The snRNA activating protein complex (SNAPc) exclusively recognizes the proximal sequence element (PSE) at snRNA promoters and recruits RNA polymerase II or III to initiate transcription. The vertebrate SNAPc consists of five subunits: SNAP190 (SNAPC4, PTFα), SNAP50 (SNAPC3, PTFβ), SNAP45 (SNAPC2, PTFδ), SNAP43 (SNAPC1, PTFγ), and SNAP19 (SNAPC5). The partial complex, termed mini-SNAPc, is composed of N-terminal third part of SNAP190, SNAP50, and SNAP43, and is fully functional for PSE-binding and snRNA transcription. SNAPc is a critical transcription factor (TF) in snRNA genes transcription, and its interaction with PSE is the first step to recruit Pol II- or Pol III-specific factors in the assembly of pre-initiation complex (PIC).

Finally, we solved the cryo-EM structure of mSNAPc#2 in complex with 35 bp human U6-1 PSE-containing sequence at the overall resolution of 3.49 Å. With the exception of some disordered regions, the atomic model of SNAP190(144-502), SNAP43(4-147), and SNAP50(28-411) are built well de novo into the other visible densities. The densities of the extreme N-terminal domain (residues 1-143) of SNAP190, the middle domain (residues 148-268) of SNAP43, and subunit SNAP19 are missing in our structure. Briefly, in DNA-binding state, SNAP50 constitutes the scaffold of mini-SNAPc architecture and it is surrounded by SNAP190(144-502) and SNAP43(4-147). The subunit of SNAP50 does not have any known homologous structure, and we divided it into three domains, namely N-terminal Lasso domain, middle imperfect β-barrel domain mainly composed of one α-helix and eight β-sheets, and C-terminal Wedge domain. However, these zinc fingers function as the structural component rather than PSE-recognition motifs, as illustrated in the structure. Unexpectedly, in SNAP190, three MYB repeats of Rb, Rc, and Rd dock into the major groove, whereas Rh and Ra mainly take part in SNAPc assembly. The first one is R445 of Rc domain, which forms hydrogen bonds with the purine groups of CG pairs at positions −62 and −61. SNAP50 recognizes the 3’ half of PSE mainly by interacting with the minor groove. Combined with three MYB repeats of SNAP190, mini-SNAPc binds tightly to PSE in a sandwich mode of “major–minor-major” groove.

> DYKDDDDKSLEVLFQGPMDVDAEREKITQEIKELERILDPGSSGSHVEISESSLESDSEADSLPSEDLDPADPPISEEERWGEASNDEDDPKDKTLPEDPETCLQLNMVYQEVIQEKLAEANLLLAQNREQQEELMRDLAGSKGTKVKDGKSLPPSTYMGHFMKPYFKDKVTGVGPPANEDTREKAAQGIKAFEELLVTKWKNWEKALLRKSVVSDRLQRLLQPKLLKLEYLHQKQSKVSSELERQALEKQGREAEKEIQDINQLPEEALLGNRLDSHDWEKISNINFEGSRSAEEIRKFWQNSEHPSINKQEWSREEEERLQAIAAAHGHLEWQKIAEELGTSRSAFQCLQKFQQHNKALKRKEWTEEEDRMLTQLVQEMRVGSHIPYRRIVYYMEGRDSMQLIYRWTKSLDPGLKKGYWAPEEDAKLLQAVAKYGEQDWFKIREEVPGRSDAQCRDRYLRRLHFSLKKGRWNLKEEEQLIELIEKYGVGHWAKIASELPHRSGSQCLSKWKIMMGKKQGL;> MAEGSRGGPTCSGVGGRQDPVSGSGGCNFPEYELPELNTRAFHVGAFGELWRGRLRGAGDLSLREPPASALPGSQAADSDREDAAVARDLDCSLEAAAELRAVCGLDKLKCLEDGEDPEVIPENTDLVTLGVRKRFLEHREETITIDRACRQETFVYEMESHAIGKKPENSADMIEEGELILSVNILYPVIFHKHKEHKPYQTMLVLGSQKLTQLRDSIRCVSDLQIGGEFSNTPDQAPEHISKDLYKSAFFYFEGTFYNDKRYPECRDLSRTIIEWSESHDRGYGKFQTARMEDFTFNDLCIKLGFPYLYCHQGDCEHVIVITDIRLVHHDDCLDRTLYPLLIKKHWLWTRKCFVCKMYTARWVTNNDSFAPEDPCFFCDVCFRMLHYDSEGNKLGEFLAYPYVDPGTFN;> HHHHHHSENLYFQGMGTPPGLQTDCEALLSRFQETDSVRFEDFTELWRNMKFGTIFCGRMRNLEKNMFTKEALALAWRYFLPPYTFQIRVGALYLLYGLYNTQLCQPKQKIRVALKDWDEVLKFQQDLVNAQHFDAAYIFRKLRLDRAFHFTAMPKLLSYRMKKKIHRAEVTEEFKDPSDRVMKLITSDVLEEMLNVHDHYQNMKHVISVDKSKPDKALSLIKDDFFDNIKNIVLEHQQWHKDRKNPSLKSKTNDGEEKMEGNSQETERCERAESLAKIKSK1,5,5-trimethylimidazolidine-2,4-dione | C6 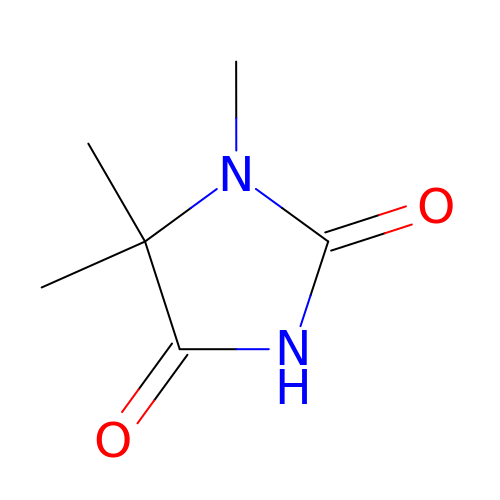H10 N2 O2 | ZNYIPTYJBRGSSL-UHFFFAOYSA-N> MGYVEIIEQPKQRGMRFRYKCEGRSAGSIPGERSTDTTKTHPTIKINGYTGPGTVRISLVTKDPPHRPHPHELVGKDCRDGFYEAELCPDRCIHSFQNLGIQCVKKRDLEQAISQRIQTNNNPFQVPIEEQRGDYDLNAVRLCFQVTVRDP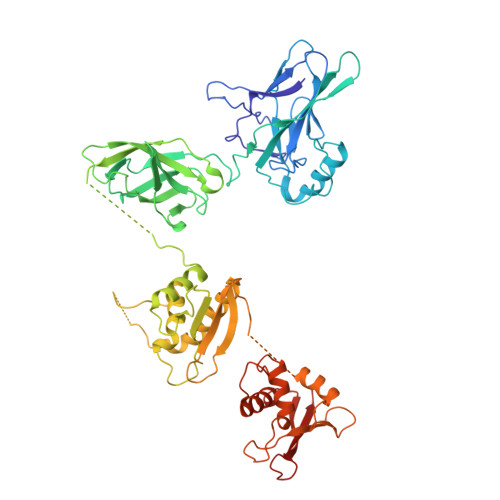SGRPLRLPPVLSHPIFDNRAPNTAELKICRVNRNSGSCLGGDEIFLLCDKVQKEDIEVYFTGPGWEARGSFSQADVHRQVAIVFRTPPYADPSLQAPVRVSMQLRRPSDRELSEPMEFQYLPDGSLSSGSSLSSPSAGAAPRVLFGEWLLGEISSGCYEGLQWLDEARTCFRVPWKHFARKDLSEADARIFKAWAVARGRWPPSSRGGGPPPEAETAERAGWKTNFRCALRSTRRFVMLRDNSGDPADQHKVYALSGSLSSDSSLSSPSALSPKPRILPWLVSQLDLGQLEGVAWVNKSRTRFRIPWKHGLRQDAQQEDFGIFQAWAEATGAYVPGRDKPDLPTWKRNFRSALNRKEGLRLAEDRSKDPHDPHKIYEFVNGLEHHHHHH>MSDNIRRSMPLFPIGIVMQLTELSARQIRYYEENGLIFPARTEGNRRLFSFHDVDKLLEIKH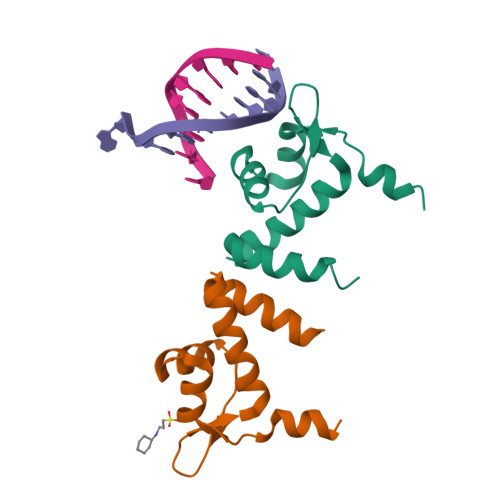LIEQGVNMAGIKQILAKAEAEP[2x]>SVVIVGKISFCPKDVLGHGAEGTIVYRGMFDNRDVAVKRILPECFSFADREVQLLRESDEHPNVIRYFCTEKDRQFQYIAIELCAATLQEYVEQKDFAHLGLEPITLLQQTTSGLAHLHSLNIVHRDLKPHNILISMPNAHGKIKAMISDFGLCKKLAVGRHSFSRRSGVPGTEGWIAPEMLSEDCKENPTYTVDIFSAGCVFYYVISEGSHPFGKSLQRQANILLGACSLDCLHPEKHEDVIARELIEKMIAMDPQKRPSAKHVLKHPFFWSLEKQLQFFQDVSDRIEKESLDGPIVKQLERGGRAVVKMDWRENITVPLQTDLRKFRTYKGGSVRDLLRAMRNKKHHYRELPAEVR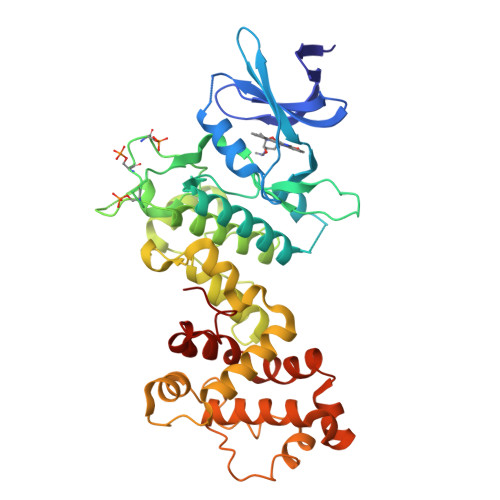ETLGSLPDDFVCYFTSRFPHLLAHTYRAMELCSHERLFQPYYFHEPP[2x]>EVKLILYHWTHSFSSQKVRLVIAEKALKCEEHDVSLPLSEHNEPWFMRLNSTGEVPVLIHGENIICEATQIIDYLEQTFLDERTPRLMPDKESMYYPRVQHYRELLDSLPMDAYTHGCILHPELTVDSMIPAYATTRIRSQIGNTESELKKLAEENPDLQEAYIAKQKRLKSKLLDHDNVKYLKKILDELEKVLDQVETELQRRNEETPEEGQQPWLCGESFTLADVSLAVTLHRLKFLGFARRNWGNGKRPNLETYYERVLKRKTFNKVLGHVNNILIS[2x]

GDAP1, a 358-amino-acid mitochondrial outer membrane (MOM) protein regulating the mitochondrial network, is highly expressed in neurons and less in Schwann cells. GDAP1 contains two domains similar to the N- and C-terminal domains of glutathione (GSH) S-transferases (GST) (GST-N and GST-C, respectively), a hydrophobic domain (HD), and a transmembrane domain (TMD). GDAP1 functions in regulating the mitochondrial network by inducing fragmentation of mitochondria without inducing apoptosis. Although the sequence identity is only ∼20%, the GDAP1 core domain shares a fold similar to canonical GST enzymes.

We determined the crystal structure of the complete human GDAP1 core domain, which shows a novel mode of dimerization within the glutathione S-transferase (GST) family. The long GDAP1-specific insertion forms an extended helix and a flexible loop. Notably, the GDAP1-specific insertion (α-loop) was present in all constructs, in contrast to a recently reported mouse GDAP1 structure. The results indicate that GDAP1 forms a unique type of homodimer mediated by a hydrophobic surface and a disulfide bridge. The main differences constitute a missing α helix between β2 and β3 and the unique helices α5 and α6 with the connecting α5-α6 loop. Variations in these regions prevent GDAP1 from forming canonical GST dimers and interacting with typical GST substrates. Contrary to predictions, we show that GDAP1 lacks helix α2. On the other hand, the catalytic Tyr9 residue of GSTA1-1 is conserved as Tyr29 in GDAP1, but Tyr29 points in another direction and makes central contacts at the GDAP1 dimer interface. A CMT-related mutation cluster of GDAP1 mainly localizes on helices α3 and α6, and less on helices α7, α8, and their connecting loops. The main cluster contains 27 residues that interact closely with each other in the crystal structure, including salt bridges, hydrogen bonds, and van der Waals interactions, forming a network of interactions.> MQKHWWHKATVYQIYPKSFMDTNGDGIGDLKGITSKLDYLQKLGVMAIWLSPVYDSPMDDNGYDIANYEAIADIFGNMADMDNLLTQAKMRGIKIIMDLVVNHTSDEHAWFIEAREHPDSSERDYYIWCDQPNDLESIFGGSAWQYDDKSDQYYLHFFSKKQPDLNWENANLRQKIYDMMNFWIDKGIGGFRMDVIDMIGKIPAQHIVSNGPKLHAYLKEMNAASFGQHDLLTVGQTWGATPEIAKQYSNPVNHELSMVFQFEHIGLQHKPEAPKWDYVKELNVPALKTIFNKWQTELELGQGWNSLFWNNHDLPRVLSIWGNTGKYREKSAKALAILLHLMRGTPYIYQGEEIGMTNYPFKDLNELDDIESLNYAKEAFTNG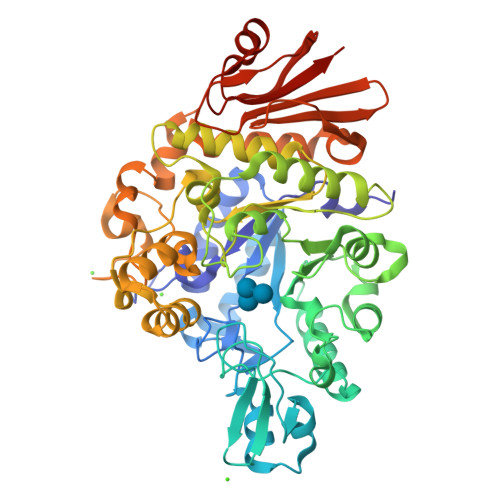KSMETIMDSIRMIGRDNARTPMQWDASQNAGFSTADKTWLPVNPNYKDINVQAALKNSNSIFYTYQQLIQLRKENDWLVDADFELLPTADKVFAYLRKVREERYLIVVNVSDQEEVLEIDVDKQETLISNTNESAALANHKLQPWDAFCIKILEHHHHHH>GFKQDIATIRGDLRTYAQDIFLAFLNKYPDERRYFKNYVGKSDQELKSMAKFGDHTEKVFNLMMEVADRATDCVPLASDANTLVQMKQHSSLTTGNFEKFFVALVEYMRASGQSFDSQSWDRFGKNLVSAL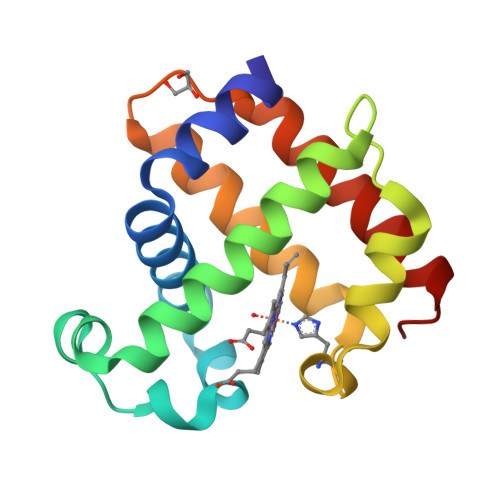SSAGMK[2x]>MASASSSQRGRSGSGNFGGGRGGGFGGNDNFGRGGNFSGRGGFGGSRGGGGYGGSGDGYNGFGNDGSNFGGGGSYNDFGNYNNQSSNFGPMKGGNFGGRSSGPYGGGGQYFAKPRNQGGYGGSSSSSSYG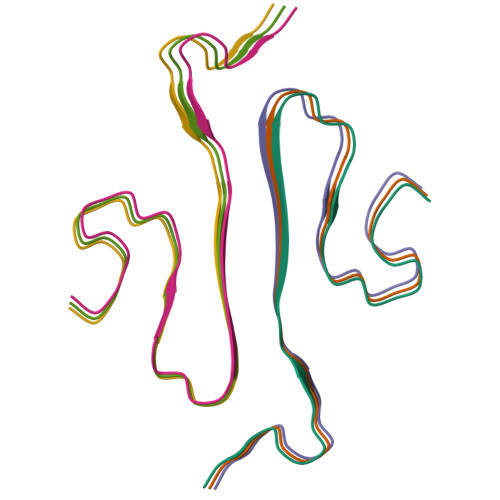SGRRF[6x]2-AMINO-5-[1-(CARBOXYLATOMETHYLCARBAMOYL)-2-NITROSOSULFANYL-ETHYL]AMINO-5-OXO-PENTANOATE | C10 H14 N4 O7 S | 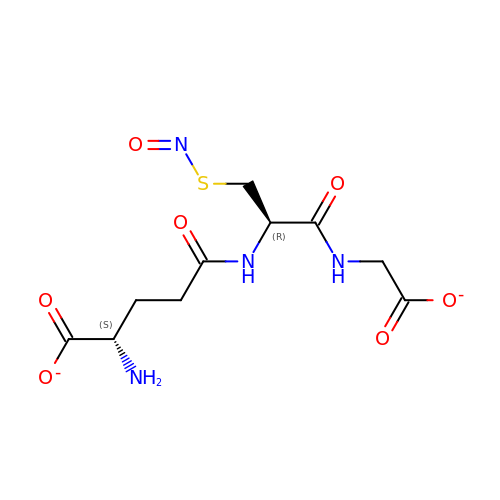HYHSBSXUHZOYLX-WDSKDSINSA-L>EAPRGRAGLESGGLLAVKHPWLSAAVRLADRDGYVLSGRLSTVEHAWVLDHVVLGTVILPGTAFVELALAAADAVGLPSVSELTIEAPLALPARGAVTLQVTVEALDATGRRGFAVHSRPDGAHDAPWTAHARGVLGAAPAAATTAWAAGAWPPAGAEPVDVTRWVEALDAWVGPAFRGVTAAWRVGRSIYADLALPEGVSERAQDFGLHPALLDAALQALLRAELGAGSSPREGIPMPFAWSDVALEARGAAALRARVEVEDASDGDQLAA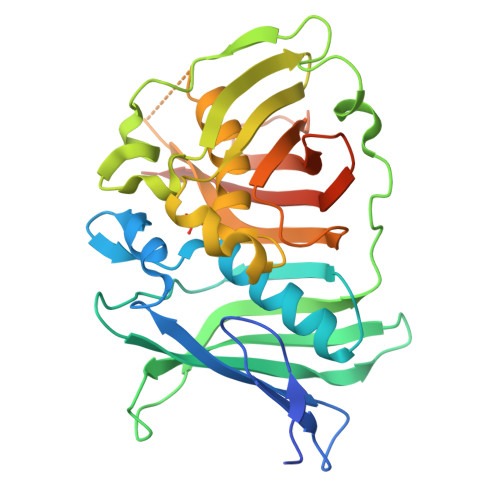SIELADAQGQPVARAGTFRARWATAEHVRKAAAGASERD[2x]>MSTQYETQGYTINNAGRRLVVDPITRIEGHMRCEVNINDQNVITNAVSCGTMFRGLEIILQGRDPRDAWAFVERICGVCTGVHALASVYAIEDAIGIKVPDNANIIRNIMLATLWCHDHLVHFYQLAGMDWIDVLDALKADPRKTSELAQSLSSWPKSSPGYFFDVQNRLKKFVEGGQLGIFRNGYWGHPQYKLPPEANLMGFAHYLEALDFQREIVKIHAVFGGKNPHPNWIVGGMPCAINIDESGAVGAVNMERLNLVQSIITRTADFINNVMIPDALAIGQFNKPWSEIGTGLSDKCVLSYGAFPDIANDFGEKSLLMPGGAVINGDFNNVLPVDLVDPQQVQEFVDHAWYRYPNDQVGRHPFDGITDPWYNPGDVKGSDTNIQQLNEQERYSWIKAPRWRGNAMEVGPLARTLIAYHKGDAATVESVDRMMSALNLPLSGIQSTLGRILCRAHEAQWAAGKLQYFFDKLMTNLKNGNLATASTEKWEPATWPTECRGVGFTEAPRGALGHWAAIRDGKIDLYQCVVPTTWNASPRDPKGQIGAYEAALMNTKMAIPEQPLEILRTLHSFNPCLACSTH[2x];>[2x]LENKPRIPVVWIHGLECTCCTESFIRSAHPLAKDVILSLISLDYDDTLMAAAGTQAEEVFEDIITQYNGKYILAVEGNPPLGEQGMF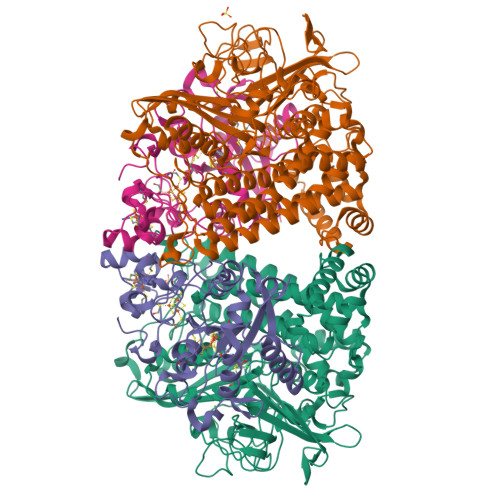CISSGRPFIEKLKRAAAGASAIIAWGTCASWGCVQAARPNPTQATPIDKVITDKPIIKVPGCPPIPDVMSAIITYMVTFDRLPDVDRMGRPLMFYGQRIHDKCYRRAHFDAGEFVQSWDDDAARKGYCLYKMGCKGPTTYNACSSTRWNDGVSFPIQSGHGCLGCAENGFWDRGSFYSRVVDIPQMGTHSTADTVGLTALGVVAAAVGVHAVASAVDQRRRHNQQPTETEHQPGNEDKQARSHHHHHH>[4x]SMESLAPFGYNKVSFKQTH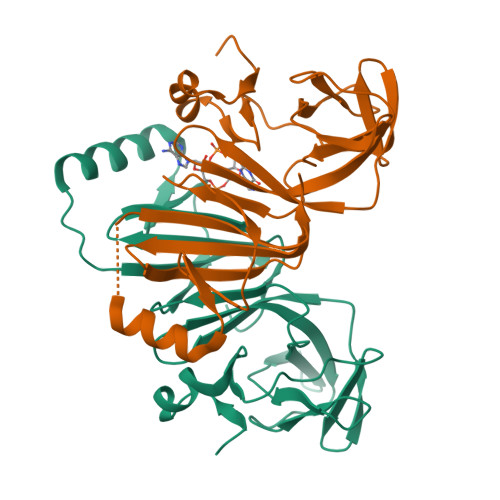HHYCGFYSLNILANIIDNVVVVNGKQYPVSDETAIDWAYDGVDTIVCEKRLVYTEREWPLHTPIYNINNQIVGLVTHGVQLSSQEYCYAVQDGFNLYNNHLTGMNLIVREKKKLIAYADREFDNKSELQIYIEETQKKNCNILGYGAILYHVNKKNAQLILHNNGLQISNSRLRKNVFGNI>MGHHHHHHMEARNMTPFTYFSLPMQKLFLRNQAAVRNKPYAKYFRSEMRVPLSAVRKIQQGPMALEDTLTPSIEDINRLLEPDFVSEESGYALLPGPMAYVQSRKFFPGCTAQMFKWWFIWHPAESERYTLWFPYAHVSNPCVHHQRLRDESLSFEERLYGNTFCASEYVGDRLMHLHIDFQQPASLGLNTDLYREAKIDGSVSALMSLADHPEVPVSLMVHLFKEVPDGMYLTSRYWVGAHPSMARFPGAEKAASLLKENGFGEAELETLAYEFAVHDMCEFNH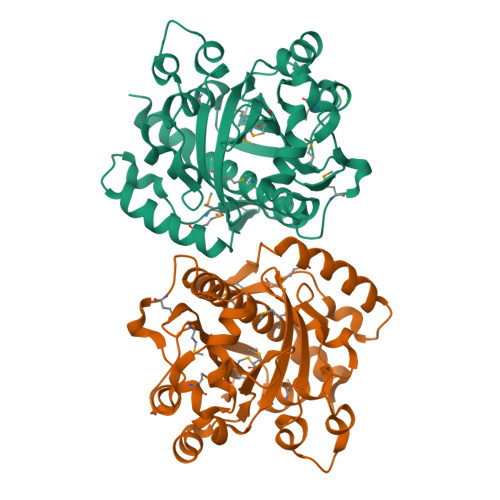LASFLPDLYREFGTPAA[2x]> SQDIVDFSQHP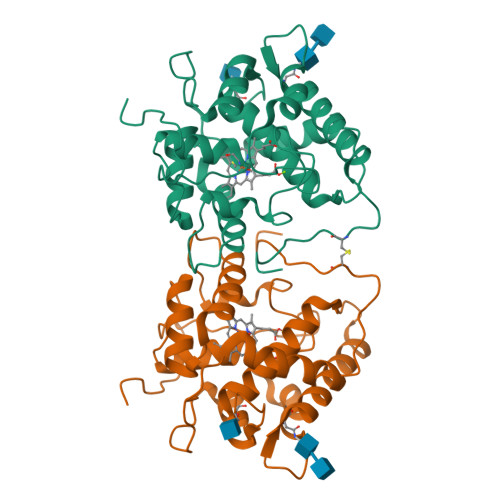WKAPGPNDLRSPCPGLNTLANHGFLPRNGRNITIPMIVQAGFDGYNVQPDILILAAKVGLLTSPEPDTFTLDDLKLHGTIEHDASLSREDFALGDNLHFNEAIFNTLANSNPGSDVYNITSAGQVLKDRLADSLARNPNVTNTGKEFTIRTLESAFYLSVMGNATTGEAPKNFVQIFFREERLPIEEGWKRSTTPITSDTLNPIAGQISEASNWKPNPDQCPWIVLSPNL> DSAAYQRTSLYGDDVVIVAAHRTPLCKSKRGN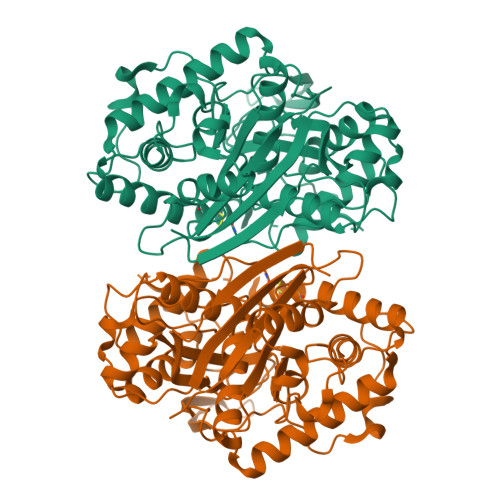FKDTYPDDLLAPVLRALIEKTNLNPSEVGDIVVGTVLAPGSQRASECRMAAFYAGFPETVAVRTVNRQCSSGLQAVADVAAAIKAGFYDIGIGAGLESMTTNPMAWEGSVNPAVKKFAQAQNCLLPMGVTSENVAQRFGVSRQEQDQAAVDSHRKAAAATAAGKFKDEIIPVKTKLVDPKTGDEKPITVSVDDGIRPTTTLASLGKLKPVFKKDGTTTAGNSSQVSDGAGAVLLMKRSVAMQKGLPVLGVFRTFAAVGVDPAIMGIGPAVAIPAAVKAAGLELDDIDLFEINEAFASQFVYCRNKLGLDPEKINVNGGAMAIGHPLGATGARCVATLLHEMKRRGKDCRFGVVSMCIGTGMGAAAVFERGDG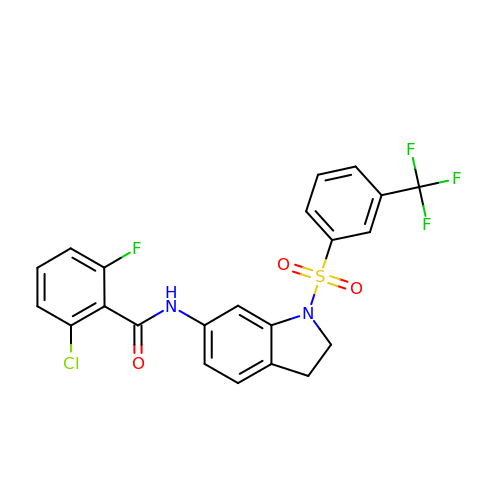2-chloro-6-fluoro-N-(1-{[3-(trifluoromethyl)phenyl]sulfonyl}-2,3-dihydro-1H-indol-6-yl)benzamide | C22 H15 Cl F4 N2 O3 S | QZUQDSDXWBNSPD-UHFFFAOYSA-N>[6x]AEIGGDHGYNATNIAAGQTSGAVTQIGPAVMGMVRRAIPNLIAFDICGVQPMNSPTGQVFALRAVYGKDPVAAGAKEAFHPMYGPDAMFSGQGAAKKFPALAASTQTTVGDIYTHFFQETGTVYLQASVQVTIDAGATDAAKLDAEIKKQMEAGALVEIAEGMATSIAELQEGFNGSTDNPWNEMGFRIDKQVIEAKSRQLKAAYSIELTQDLRAVHGMDADAELSGILATEIMLEINREVVDWINYSAQVGKSGMTLTPGSKAGVFDFQDPIDIRGARWAGESFKALLFQIDKEAVEIARQTGRGEGNFIIASRNVVNVLASVDTGISYAAQGLATGFSTDTTKSVFAGVLGGKYRVYIDQYAKQDYFTVGYKGPNEMDAGIYYAPYVALTPLRGSDPKNFQPVMGFKTRYGIGINPFAESAAQAPASRIQSGMPSILNSLGKNAYFRRVYVKGI;>MTFTVDITPKTPTGVIDETKQFTATPSGQTGGGTITYAWSVDNVPQDGAEATFSYVLKGPAGQKTIKVVATNTLSEGGPETAEATTTITVKNKTQTTTLAVTPASPAAGVIGTPVQFTAALASQPDGASATYQWYVDDSQVGGETNSTFSYTPTTSGVKRIKCVAQVTATDYDALSVTSNEVSLTVNKKTMNPQVTLTPPSINVQQDASATFTANVTGAPEEAQITYSWKKDSSPVEGSTNVYTVDTSSVGSQTIEVTATVTAADYNPVTVTKTGNVTVTAKVAPEPEGELPYVHPLPHRSSAYIWCGWWVMDEIQKMTEEGKDWKTDDPDSKYYLHRYTLQKMMKDYPEVDVQESRNGYIIHKTALETGIIYTYP[2x]

The outer surface of the head is decorated with the highly antigenic outer capsid protein Hoc and the small outer capsid protein Soc. The 376-residue Hoc is a monomeric fiber consisting of a string of four domains connected by flexible short linkers, of which the three N-terminal domains have an immunoglobulin (Ig)-like fold. The Hoc subunits bind near the centers of gp23* capsomers, one per hexon, and have only a marginal effect on the capsid stability. Each T4-Hoc fiber attaches randomly to the center of gp23* hexameric capsomers in one of the six possible orientations, though at the vertex-proximal hexamers that deviate from 6-fold symmetry, Hoc binds in two preferred orientations related by 180° rotation.

The atomic model consisting of the vertex-proximal gp23* hexamer and two C-terminal domains of Hoc corresponding to the preferred orientations was refined against the 3.3 Å-resolution cryo-EM reconstruction of the isometric T4 capsid (EMDB-8661) by adjusting the structure into the density using the Coot program, and refinement in the real space was carried out using the phenix.real_space_refine program. During refinement, the two Hoc C-terminal domains in the model were treated as two alternative orientations of the same domain contributing to the cryo-EM density. The refinement of the occupancies for the two Hoc orientations using the Phenix software resulted in occupancy values of 0.4 and 0.33 for the preferred orientations 1 and 2, respectively. Since the isometric capsid reconstruction is of a higher resolution and shows stronger density for the Hoc C-terminal domain, here we describe the Hoc-gp23* structure refined against the isometric map. The C-terminal domain of T4 Hoc contains a four-stranded β-sheet and a three-helix bundle on top of the β-sheet. The Hoc C-terminal domain, in both the preferred orientations, interacts with six gp23* subunits with an interface area of ~1200 Å2. In the preferred orientation 1, which shows the highest occupancy, Hoc interacts most extensively with the gp23* subunit A, which is the closest to the pentameric vertex. The residues Arg300 and His299 of the Hoc C-terminal domain, which are located in the loop between β-strands 1 and 2, are involved in charge interactions with the Asp336 of the gp23* subunit A, thus reinforcing the Hoc attachment to the capsid. The Hoc molecule in the alternative preferred orientation 2 is rotated by 180° around the capsomer axis with respect to Hoc in orientation 1. In this orientation, Hoc shows the most extensive interactions with the gp23* subunit D, which is related to subunit A by the 180° rotation.> GNAS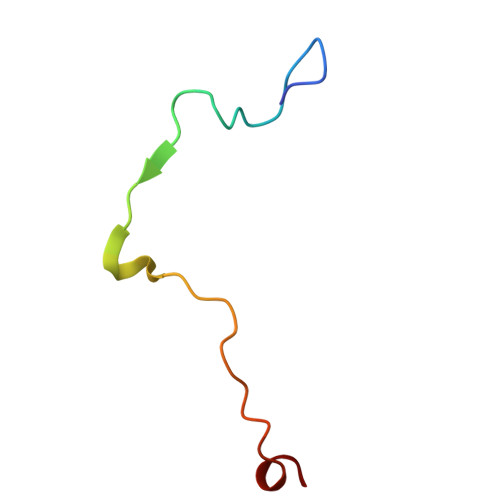SIVQTINVTGDGNVFKPSAETSSTAVPSLSLSPGMLN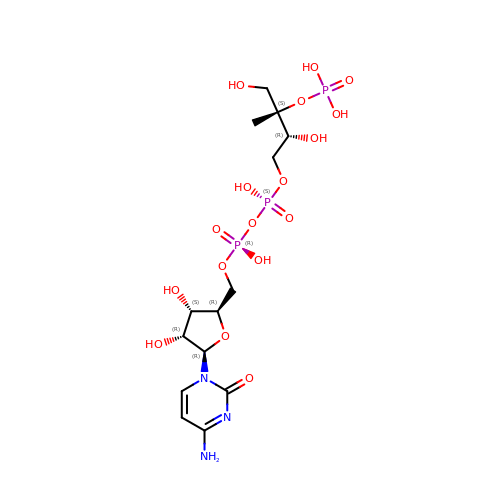4-DIPHOSPHOCYTIDYL-2-C-METHYL-D-ERYTHRITOL 2-PHOSPHATE | C14 H26 N3 O17 P3 | HTJXTKBIUVFUAR-XHIBXCGHSA-N> GPGSEFELPLPEGWEEARDFDGKV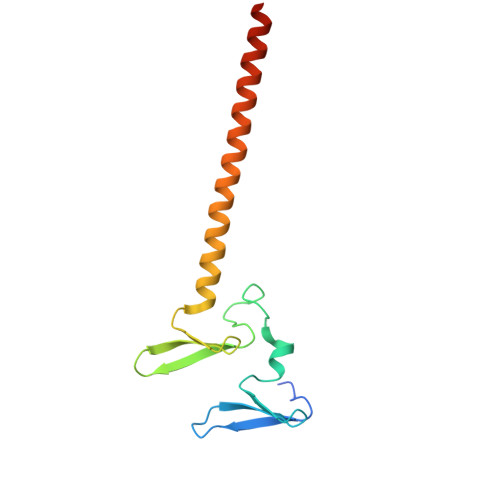YYIDHRNRTTSWIDPRDRYTKPLTFADCISDELPLGWEEAYDPQVGDYFIDHNTKTTQIEDPRVQWRREQEHMLKDYLVVAQEALSAQKEIYQVKQQRLELAQQEYQQLH> RPFSVAEVEALVEAV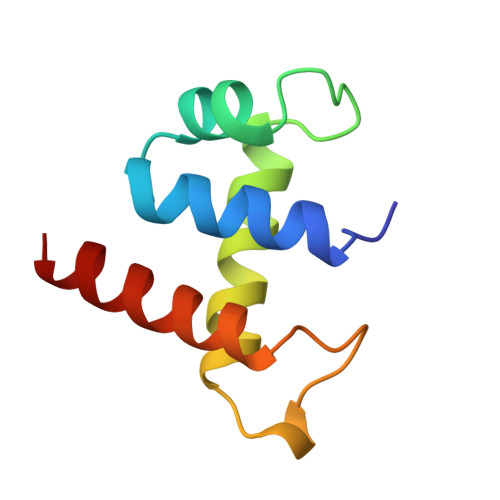EHLGTGRWRDVKMRAFDNADHRTYVDLKDKWKTLVHTASIAPQQRRGEPVPQDLLDRVLAAHAYWSQQ> MIPSITAYSKNGLKIEFTFERSNTNPSVTVITIQASNSTELDMTDFVFQAAVPKTFQLQLLSPSSSVVPAFNTGTIT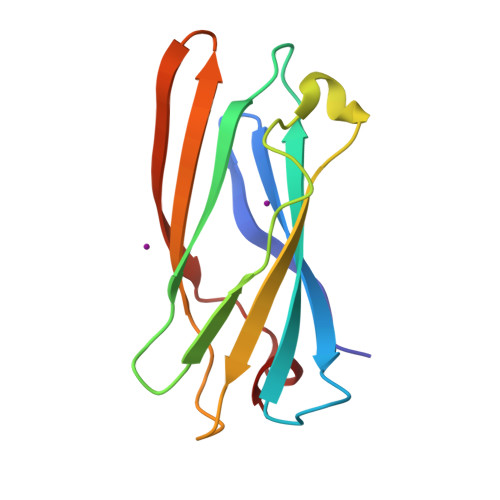QVIKVLNPQKQQLRMRIKLTYNHKGSAMQDLAEVNNFPPQSWQ> MEDINFSSLAPRHGTRPFMGTWSDIGTSQLNGGAFNWSSLWSGLKNFGSTLKTYGSKAWNSTTGQALRDKLKEQNFQQKVVDGLASGINGVVDLANQAVQRQINSRLDPVPPAGSVEMPQVEEELPPLDKRGEKRPR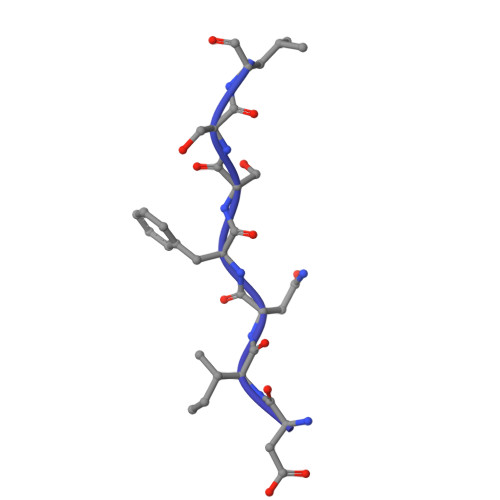PDAEETLLTHTDEPPPYEEAVKLGLPTTRPIAPLATGVLKPESNKPATLDLPPPASRPSTVAKPLPPVAVARARPGGSARPHANWQSTLNSIVGLGVQSVKRRRCY> SNSFEVSSLPDANGKNHITAVKGDAKIPVDKIELYMRGKASGDLDSLQAEYNSLKDARISSQKEFAKDPNNAKRMEVLEKQIHNIERSQDMARVLEQAGIVNTASNNSMIMDKLLDSAQGATSANRKTSVVVSGPNGNV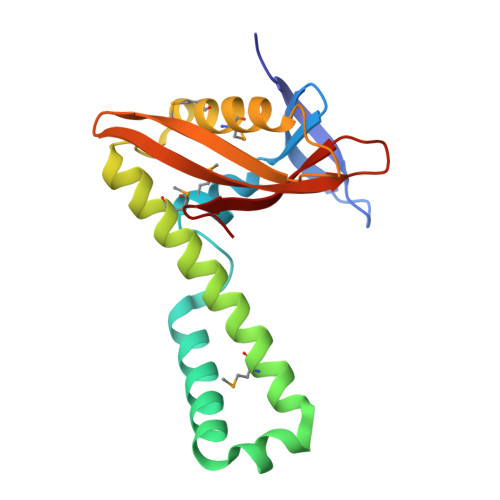RIYATWTILPDGTKRLSTVTGTFK>MGAAPDSHQLAKALAEAADVGAQMIKLVGLRELSEAERQLRSLVVALMQEVFTEFFPGCVVHPFGSSINSFDVHGCDLDLFLDLGDLEEPQPVPKLPPASPLLEDREEGDLGKASELAETPKEEKAEGAAMLELVGSILRGCVPGVYRVQTVPSARRPVVKFAHRPSGLHGDVSLSNRLALHNSRFLSLCSELDGRVRPLVYTLRAWAQGRGLSGSGPLLSNYALTLLVIYFLQTRDPPVLPTVSQLTQKAGEGEQVEVDGWDCSFPRDASRLEPSINVEPLSSLLAQFFSAVSSWDLRGSLLSLREGQALPVAGGLPSNLWEGLRLGPLNLQDPFDLSHNVAANVTSRVAGRLQNCCRAAANYCRSLQYQRRSSRGRDWGLLPLLQPSSPSSLLSATPIPLPLAPFTQLTAALVQVFREALGCHIEQATKRTRSEGGGTGQGEAGKGASLPSSASWRCALWHRVWQGRRRARRRLQQQTKEGAGGGAGTRAGWLATEAQVTQELKGLSGGEERPETEPLLSFVASVSPADRMLTVTPLQDPQGLFPDLHHFLQVFLPQAIRHLKLEHHHHHH[2x]

After transcription, the 3′-end is oligo-uridylylated by a terminal uridylyltransferase, TUT1 (TUTase6)910, one of the members of the non-canonical nucleotidyltransferases. TUT1 is composed of N-terminal Zn-finger, RRM, palm, fingers and KA-1 domains. The C-terminal region of TUT1 is a previously unidentified RNA-binding domain, and it was named the KA-1 domain. Thus, the present structural and biochemical studies have demonstrated that TUT1 acts as a U6 snRNA-specific terminal uridylyltransferase.

The truncated TUT1 (TUT1_ΔN) was overexpressed in Escherichia coli, purified and crystallized. The form-I and -II crystals belong to the space groups P21212, and P21, respectively. The form-I TUT1_ΔN structure complexed with UTP (soaked in) was initially solved by the single isomorphous replacement with anomalous scattering (SIRAS) method, using the protein complexed with UTP in the presence of BaCl2. Subsequently, the structure was modelled and refined to an R factor of 24.6% (Rfree of 29.4%), using reflections up to 2.95 Å resolution. The nucleotide is located in the cleft between the palm and fingers domains.> PVENLEKEITAIVAEVTELDE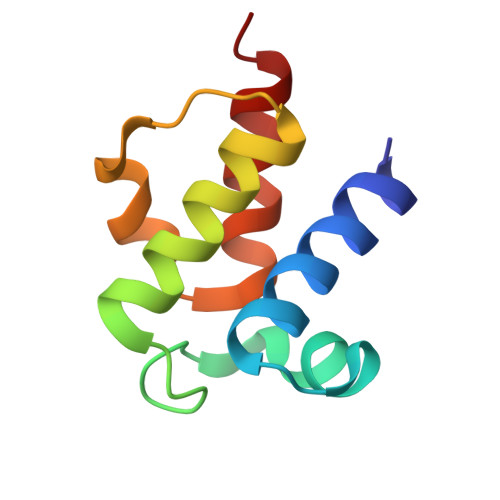NEIWEKRDADFFKDLEIDSLLALEILALIEKKFKVQIPEEKLVDITSLNATIEMTRSTLEGK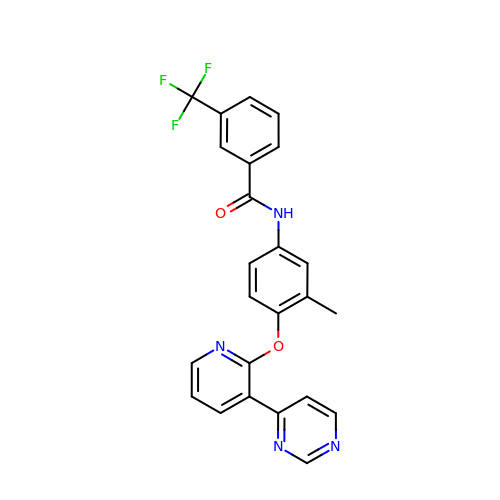N-{3-methyl-4-[(3-pyrimidin-4-ylpyridin-2-yl)oxy]phenyl}-3-(trifluoromethyl)benzamide | C24 H17 F3 N4 O2 | OHDDQNLJTAKXQT-UHFFFAOYSA-N>[2x]MESSTYQERADELVVKIKDMFNALGDGDISPSAYDTAWVARLATISSDGSEKPRFPQALNWVFNNQLQDGSWGIESHFSLCDRLLNTTNSVIALSVWKTGHSQVQQGAEFIAENLRLLNEEDELSPDFQIIFPALLQKAKALGINLPYDLPFIKYLSTTREARLTDVSAAADNIPANMLNALEGLEEVIDWNKIMRFQSKDGSFLSSPASTACVLMNTGDEKCFTFLNNLLDKFGGCVPCMYSIDLLERLSLVDNIEHLGIGRHFKQEIKGALDYVYRHWSERGIGWGRDSLVPDLNTTALGLRTLRMHGYNVSSDVLNNFKDENGRFFSSAGQTHVELRSVVNLFRASDLAFPDERAMDDARKFAEPYLREALATKISTNTKLFKEIEYVVEYPWHMSIPRLEARSYID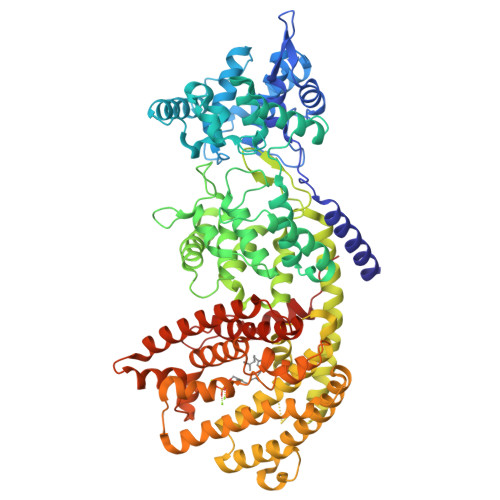SYDDNYVWQRKTLYRMPSLSNSKCLELAKLDFNIVQSLHQEELKLLTRWWKESGMADINFTRHRVAEVYFSSATFEPEYSATRIAFTKIGCLQVLFDDMADIFATLDELKSFTEGVKRWDTSLLHEIPECMQTCFKVWFKLMEEVNNDVVKVQGRDMLAHIRKPWELYFNCYVQEREWLEAGYIPTFEEYLKTYAISVGLGPCTLQPILLMGELVKDDVVEKVHYPSNMFELVSLSWRLTNDTKTYQAEKARGQQASGIACYMKDNPGATEEDAIKHICRVVDRALKEASFEYFKPSNDIPMGCKSFIFNLRLCVQIFYKFIDGYGIANEEIKDYIRKVYIDPIQVGSHHHHHH>[2x]MENTENSVDSKSIKNLEPKIIHGSESMDSGISLDNSYKMDYPEMGLCIIINNKNFHKS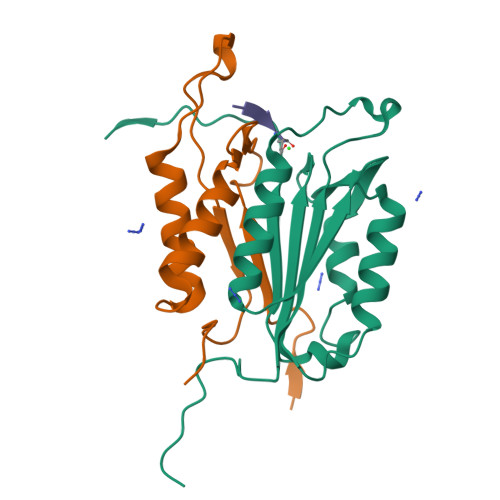TGMTSRSGTDVDAANLRETFRNLKYEVRNKNDLTREEIVELMRDVSKEDHSKRSSFVCVLLSHGEEGIIFGTNGPVDLKKITNFFRGDRCRDLTGKPKLFIIQACRGTELDCGIETD;>[2x]SGVDDDMACHKIPVEADFLYAYSTAPGYYSWRNSKDGSWFIQSLCAMLKQYADKLEFMHILTRVNRKVATEFESFSFDATFHAKKQIPCIVSMLTKELYFYHH>GSHMTGSEGTAPDIRVPVLIVGGGPAGLTAALALSRYGVPHLLVNRHHGTAHTPRAHLLNQRTGEIFRDLGIADRVEAHATPGHLMANHVFMSTFAGPEVARIGAYGNGPDRIGEYRAASPSGLCNLPQHLLEPLLVEAVQEACVGQLRFGHEFVSLEQDEHGVTSRITDRRTGRDYTVRSDYLIGADGARSRVLAQLGIALDGATGIARAVTTWFEADLSRYSAHRPALLYMGAVPGSPPADGRVFVSLRPWTEWLHLTFPPPTADVDVEDHEAVRAGIRESIGDPTVDVTIKNVSAWEVNSAVAPRYASGRVFCVGDAVHQNPPTNGLGLNSAVADSFNLCWKLKLALEGLAGPGLLDTYHDERQPVGRQIVDRAFRSMVDLIGIPQALGFTEGQSPEEQWRLLDTLHEDTEEARQRRAALAAATAAIHGQANAHGVELGYRYRTGALVPDGTPEPADERDPELYYRATTWPGARLPHAWLENGRHRCSTLDVTGRGRFTLLTGPGGEPWRDAARDAALDTGVEVAVLPIGAGGGPRDPYGTWAELREVEESGAVLVRPDGHVAWRARDHGHAKELPEVMARVLHQPDPAA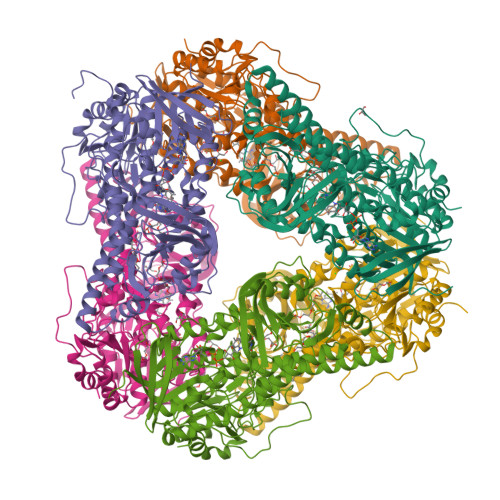RRTGGPGA[6x]>[4x]MEIAFLLNGETRRVRIEDPTQSLLELLRAEGLTGTKEGCNEGDCGACTVMIRDAAGSRAVNACLMMLPQIAGKALRTIEGIAAPDGRLHPVQQAMIDHHGSQCGFCTPGFIVSMAAAHDRDRKDYDDLLAGNLCRCTGYAPILRAAEAAAGEPPADWLQADAAFTLAQLSSGVRGQT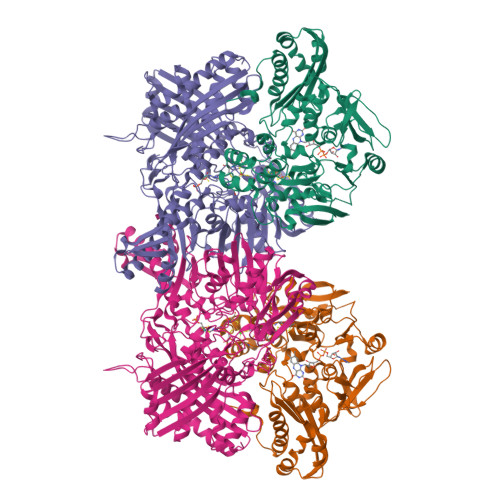APAFLPETSDALADWYLAHPEATLIAGGTDVSLWVTKALRDLPEVAFLSHCKDLAQIRETPDGYGIGAGVTIAALRAFAEGPHPALAGLLRRFASEQVRQVATIGGNIANGSPIGDGPPALIAMGASLTLRRGQERRRMPLEDFFLEYRKQDRRPGEFVESVTLPKSAPGLRCYKLSKRFDQDISAVCGCLNLTLKGSKIETARIAFGGMAGVPKRAAAFEAALIGQDFREDTIAAALPLLAQDFTPLSDMRASAAYRMNAAQAMALRYVRELSGEAVAVLEVMP;>MSVGKPLPHDSARAHVTGQARYLDDLPCPANTLHLAFGLSTEASAAITGLDLEPVRESPGVIAVFTAADLPHDNDASPAPSPEPVLATGEVHFVGQPIFLVAATSHRAARIAARKARITYAPRPAILTLDQALAADSRFEGGPVIWARGDVETALAGAAHLAEGCFEIGGQEHFYLEGQAALALPAEGGVVIHCSSQHPSEIQHKVAHALGLAFHDVRVEMRRMGGGFGGKESQGNHLAIACAVAARATGRPCKMRYDRDDDMVITGKRHDFRIRYRIGADASGKLLGADFVHLARCGWSADLSLPVCDRAMLHADGSYFVPALRIESHRLRTNTQSNTAFRGFGGPQGALGMERAIEHLARGMGRDPAELRALNFYDPPERGGLSAPPSPPEPIATKKTQTTHYGQEVADCVLGELVTRLQKSANFTTRRAEIAAWNSTNRTLARGIALSPVKFGISFTLTHLNQAGALVQIYTDGSVALNHGGTEMGQGLHAKMVQVAAAVLGIDPVQVRITATDTSKVPNTSATAASSGADMNGMAVKDACETLRGRLAGFVAAREGCAARDVIFDAGQVQASGKSWRFAEIVAAAYMARISLSATGFYATPKLSWDRLRGQGRPFLYFAYGAAITEVVIDRLTGENRILRTDILHDAGASLNPALDIGQIEGAYVQGAGWLTTEELVWDHCGRLMTHAPSTYKIPAFSDRPRIFNVALWDQPNREETIFRSKAVGEPPFLLGISAFLALHDACAACGPHWPDLQAPATPEAVLAAVRRAEGRA[4x]> MFKTEFEFPEELKTKLQEHINYFPKKRQAILLCLHEIQNYYGYIPPESLKPLADMLELPLNHVEGVVAF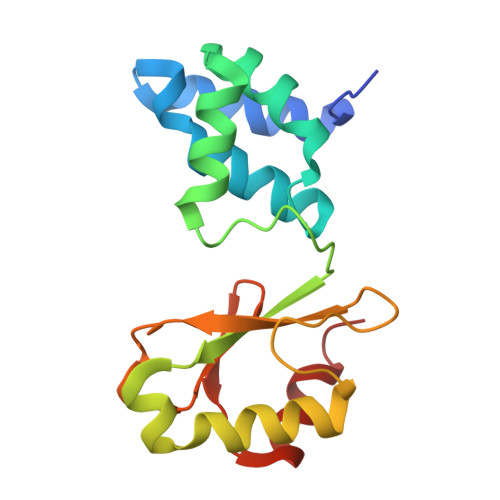YDMFDREDKAKYRIRVCVSIVCHLMGTNKLLKALENILGIKPGEVTPDGKFKIVPVQCLSACSEAPVFMVNDDEYKFESEVQLNEILSRYT>MMERLIGSTPIVRLDSIDSRIALKLEKNNPGGSVKDRPALFMILDAEKRGLLKNGIVEPTSGNMGIAIAMIGAKRGHRVILTMPETMSVERRKVLKMLGAELVLTPGELGMKGAVEKALEISRETGAHMLNQFENPYNVYSHQFTTGPEILKQMDYQIDAFVAGVGTGGTISGVGRVLKGFFGNGVKIVAVEPAKSPVLSGGQPGKHAIQGIGAGFVPKILDRSVIDEVITVEDEEAYEMARYLAKKEGLLVGISSGANVAAALKVAQKLGPDARVVTVAPD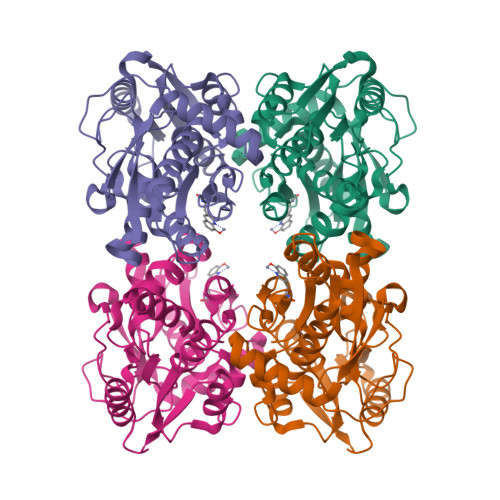HAERYLSIL[2x]> KTAQQLKYIKDSIKTIPDYPKAGILFRDVTSLLENPKAYSASIELLSEHYSESGVTKVVGTEARGFLFGAPVALALGVGFVPVRKPGKLPRETI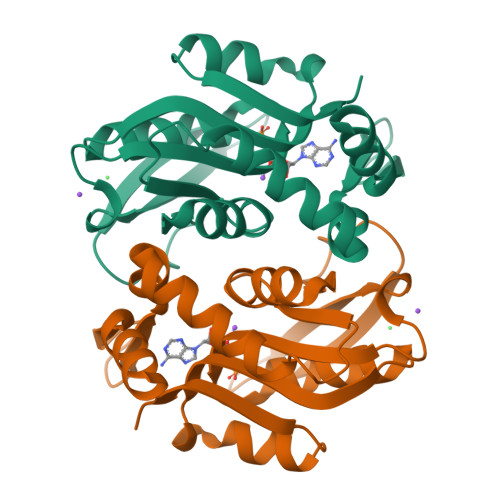SESYELEYGTDTLEIHTDSIQPGDKVLVVDDLLATGGTIEATVKLIRRLGGEVVHAAFIINLPELGGEARLTQQGIHCYSLVSFDGH> DEEEIQKAIEELLRKGVSEEEAAIIIVQRFNVAVVVVVQDERQGKHISEYIRRYIPEADVILF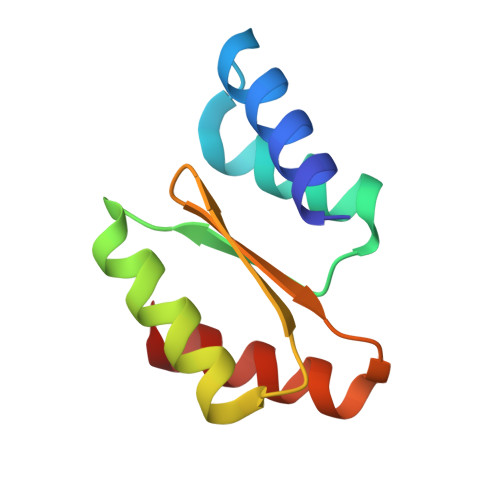ANLVVIKVETHELSTRVWEAAQKAY>[2x]SGDMADAFGDELFSVFEGDSTTAAGTKKDKEKDKGKWKGPPGSADKAGKRFDGKLQSESTNNGKNKRDVDFEGTDEPIFGKKPRIEESITEDLSLADLMPRVKVQSVETVEGCTHEVALPAEEDYLPLKPRVGKAAKEYPFILDAFQREAIQCVDNNQSVLVSAHTSAGKTVCAEYAIALALREKQRVIFTSPIKALSNQKYREMYEEFQDVGLMTGDVTINPTASCLVMTTEILRSMLYRGSEVMREVAWVIFDEIHYMRDSERGVVWEETIILLPDNVHYVFLSATIPNARQFAEWICHLHKQPCHVIYTDYRPTPLQHYIFPAGGDGLHLVVDENGDFREDNFNTAMQVLRDAGDLAKGDQKGRKGGTKGPSNVFKIVKMIMERNFQPVIIFSFSKKDCEAYALQMTKLDFNTDEEKKMVEEVFSNAIDCLSDEDKKLPQVEHVLPLLKRGIGIHHGGLLPILKETIEILFSEGLIKALFATETFAMGINMPARTVLFTNARKFDGKDFRWISSGEYIQMSGRAGRRGMDDRGIVILMVDEKMSPTIGKQLLKGSADPLNSAFHLTYNMVLNLLRVEEINPEYMLEKSFYQFQHYRAIPGVVEKVKNSEEQYNKIVIPNEESVVIYYKIRQQLAKLGKEIEEYIHKPKYCLPFLQPGRLVKVKNEGDDFGWGVVVNFSKKSNVKPNSGELDPLYVVEVLLRCSKESLKNSATEAAKPAKPDEKGEMQVVPVLVHLLSAISSVRLYIPKDLRPVDNRQSVLKSIQEVQKRFPDGIPLLDPIDDMGIQDQGLKKVIQKVEAFEHRMYSHPLHNDPNLETVYTLCEKKAQIAIDIKSAKRELKKARTVLQMDELKCRKRVLRRLGFATSSDVIEMKGRVACEISSADELLLTEMMFNGLFNDLSAEQATALLSCFVFQENSSEMPKLTEQLAGPLRQMQECAKRIAKVSAEAKLEIDEETYLSSFKPHLMDVVYTWA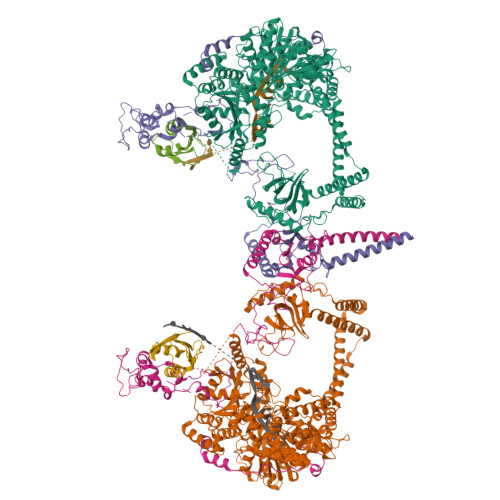TGATFAHICKMTDVFEGSIIRCMRRLEELLRQMCQAAKAIGNTELENKFAEGITKIKRDIVFAASLYL;>SGDMAAEVYFGDLELFEPFDHPEESIPKPVHTRFKDDDGDEEDENGVGDAELRERLRQCEETIEQLRAENQELKRKLNILTRPSGILVNDTKLDGPILQILFMNNAISKQYHQEIEEFVSNLVKRFEEQQKNDVEKTSFNLLPQPSSIVLEEDHKVEESCAIKNNKEAFSVVGSVLYFTNFCLDKLGQPLLNENPQLSEGWEIPKYHQVFSHIVSLEGQEIQVKAKRPKPHCFNCGSEEHQMKDCPMPRNAARISEKRKEYMDACGEANNQNFQQRYHAEEVEERFGRFKPGVISEELQDALGVTDKSLPPFIYRMRQLGYPPGWLKEAELENSGLALYDGKDGTDGETEVGEIQQNKSVTYDLSKLVNYPGFNISTPRGIPDEWRIFGSIPMQACQQKDVFANYLTSNFQAPGVKSGGAVDEDALTLEELEEQQRRIWAALEQAESVNSDSDVPVDTPLTGNSVASSPCPNELDLPVPEGKTSEKQTLDEPEVPEIFTKKSEAGHASSPDSEVTSLCQKEKAELAPVNTEGALLDNGSVVPNCDISNGGSQKLFPADTSPSTATKIHSPIPDMSKFATGITPFEFENMAESTGMYLRIRSLLKNSPRNQQKNKKASE[2x];>SGDEADRTLFVGNLETKVTEELLFELFHQAGPVIKVKIPKDKDGKPKQFAFVNFKHEVSVPYAMNLLNGIKLYGRPIKIQFRS[2x]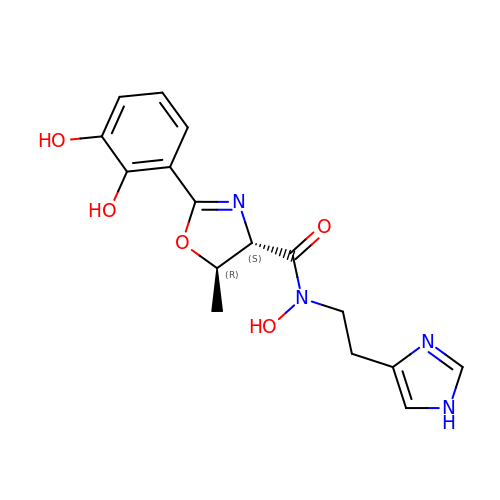(4~{S},5~{R})-2-[2,3-bis(oxidanyl)phenyl]-~{N}-[2-(1~{H}-imidazol-4-yl)ethyl]-5-methyl-~{N}-oxidanyl-4,5-dihydro-1,3-oxazole-4-carboxamide | C16 H18 N4 O5 | FCWIGDCVHNNXFS-RNCFNFMXSA-N>RNRREEILQSLALMLESSDGSQRITTAKLAASVGVSEAALYRHFPSKTRMFDSLIEFIEDSLITRINLILKDEKDTTARLRLIVLLLLGFGERNPGLTRILTGHALMFEQDRLQGRINQLFER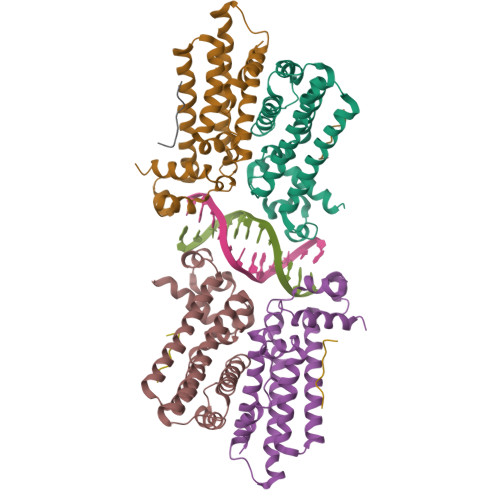IEAQLRQVMREKRMREGEGYTTDETLLASQILAFCEGMLSRFVRSEFKYRPTDDFDARWPLIAAQLQ[4x];>LDIPAFLR[4x]> PKHEFSVDMTC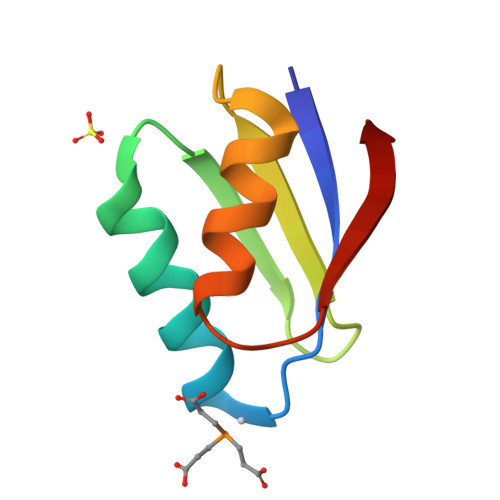GGCAEAVSRVLNKLGGVKYDIDLPNKKVCIESEHSMDTLLATLKKTGKTVSYLGLE>[2x]GKAVIAIHGGAGAISRAQMSLQQELRYIEALSAIVETGQKMLEAGESALDVVTEAVRLLEECPLFNAGIGAVFTRDETHELDACVMDGNTLKAGAVAGVSHLRNPVLAARLVMEQSPHVMMIGEGAENFAFARGMERVSPEIFSTSLRYEQLLAARKEGATVLDHSGAPLDEKQKMGAVGAVA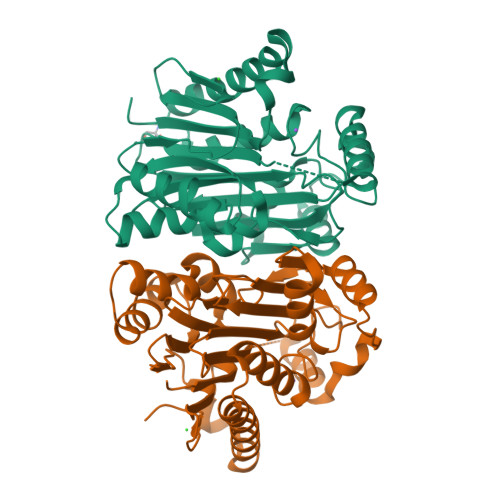LDLDGNLAAATSTGGMTNKLPGRVGDSPLVGAGCYANNASVAVSCTGTGEVFIRALAAYDIAALMDYGGLSLAEACERVVMEKLPALGGSGGLIAIDHEGNVALPFNTEGMYRAWGYAGDTPTTGIYREKGDTVATQ>MFNDRVIVKKSPLGGYGVFARKSFEKGELVEECLCIVRHNDDWGTALEDYLFSRKNMSAMALGFGAIFNHSKDPNARHELTAGLKRMRIFTIKPIAIGEEITISYGDDYWLSRPRL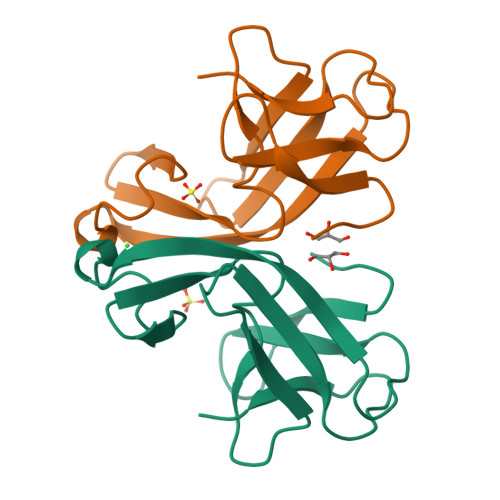TQN[2x]> GSGFTSKDTYLSHFNPRDYLEKYYKFGSRHSAESQILKHLLKNLFKIFCLDGVKGDLLIDIGSGPTIYQLLSACESFKEIVVTDYSDQNLQELEKWLKKEPAAFDWSPVVTYVCDLEGNRVKGPEKEEKLRQAVKQVLKCDVTQSQPLGAVPLPPADCVLSTLCLDAACPDLPTYCRALRNLGSLLKPGGFLVIMDALKSSYYMIGEQKFSSLPLGRE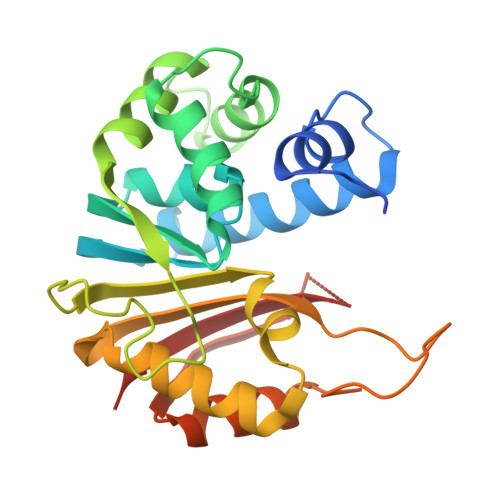AVEAAVKEAGYTIEWFEVISQSYSSTMANNEGLFSLVARKL> RLQSET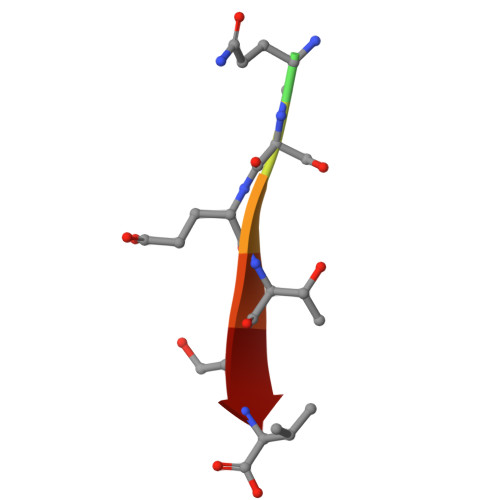SV> GSSST;> GLGQMLESMIDNTVRETVGAATSRDALPNTEASGPTHSKEIPALTAVETGATNPLVPSDTVQTRHVVQHRSRSESSIESFFARGACVTIMTVDNPASTTNKDKLFAVWKITYKDTVQLRRKLEFFTYSRFDMELTFVVTANFTETNNGHALNQVYQIMYVPPGAPVPEKWDDYTWQTSSNPSIFYTYGTAPARISVPYVGISNAYSHFYDGFSKVPLKDQSAALGDSLYGAASLNDFGILAVRVVNDHNPTKVTSKIRVYLKPKHIRVWCPRPPRAVAYYGPGVDYKDGTLTPLSTKDLTTY;> SPNIEACGYSDRVLQLTLGNSTITTQEAANSVVAYGRWPEYLRDSEANPVDQPTEPDVAACRFYTLDTVSWTKESRGWWWKLPDALRDMGLFGQNMYYHYLGRSGYTVHVQCNASKFHQGALGVFAVPEMCLAGDSNTTTMHTSYQNANPGEKGGTFTGTFTPDNNQTSPARRFCPVDYLLGNGTLLG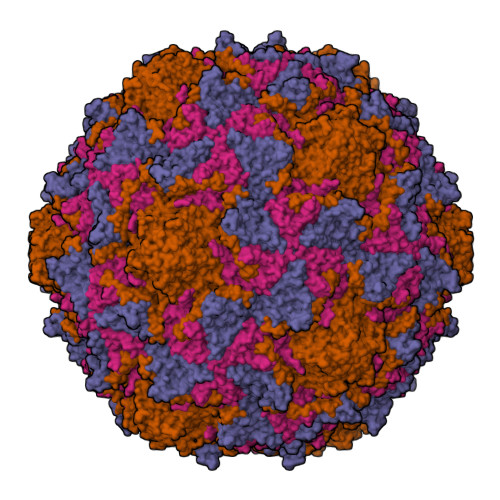NAFVFPHQIINLRTNNCATLVLPYVNSLSIDSMVKHNNWGIAILPLAPLNFASESSPEIPITLTIAPMCCEFNGLRNITLPRLQ;> GLPVMNTPGSNQYLTADNFQSPCALPEFDVTPPIDIPGEVKNMMELAEIDTMIPFDLSATKKNTMEMYRVRLSDKPHTDDPILCLSLSPASDPRLSHTMLGEILNYYTHWAGSLKFTFLFCGSMMATGKLLVSYAPPGADPPKKRKEAMLGTHVIWDIGLQSSCTMVVPWISNTTYRQTIDDSFTEGGYISVFYQTRIVVPLSTPREMDILGFVSACNDFSVRLLRDTTHIEQKALAQ;> GAQVSSQKVGAHENSNRAYGGSTINYTTINYYRDSASNAASKQDFSQDPSKFTEPIKDVLIKTAPMLN> MNTINIAKNDFSDIELAAIPFNTLADHYGERLAREQLALEHESYEMGEARFRKMFERQLKAGEVADNAAAKPLITTLLPKMIARINDWFEEVKAKRGKRPTAFQFLQEIKPEAVAYITIKTTLACLTSADNTTVQAVASAIGRAIE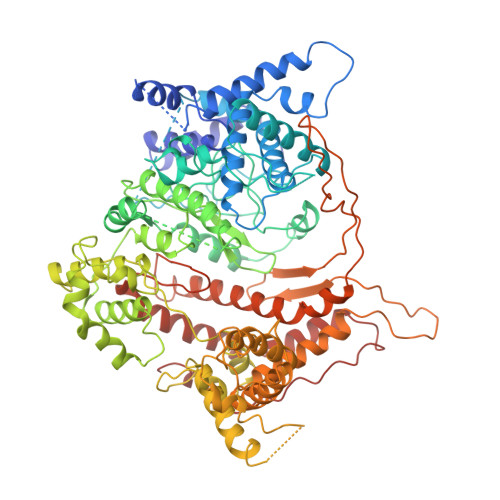DEARFGRIRDLEAKHFKKNVEEQLNKRVGHVYKKAFMQVVEADMLSKGLLGGEAWSSWHKEDSIHVGVRCIEMLIESTGMVSLHRQNAGVVGQDSETIELAPEYAEAIATRAGALAGISPMFQPCVVPPKPWTGITGGGYWANGRRPLALVRTHSKKALMRYEDVYMPEVYKAINIAQNTAWKINKKVLAVANVITKWKHSPVEDIPAIEREELPMKPEDIDMNPEALTAWKRAAAAVYRKDKARKSRRISLEFMLEQANKFANHKAIWFPYNMDWRGRVYAVSMFNPQGNDMTKGLLTLAKGKPIGKEGYYWLKIHGANCAGVDKVPFPERIKFIEENHENIMACAKSPLENTWWAEQDSPFCFLAFCFEYAGVQHHGLSYNCSLPLAFDGSCSGIQHFSAMLRDEVGGRAVNLLPSETVQDIYGIVAKKVNEILQADAINGTDNEVVTVTDENTGEISEKVKLGTKALAGQWLAYGVTRSVTKRSVMTLAYGSKEFGFRQQVLEDTIQPAIDSGKGLMFTQPNQAAGYMAKLIWESVSVTVVAAVEAMNWLKSAAKLLAAEVKDKKTGEILRKRSAVHWVTPDGFPVWQEYKKPIQTRLNLMFLGQFRLQPTINTNKDSEIDAHKQESGIAPNFVHSQDGSHLRKTVVWAHEKYGIESFALIHDSFGTIPADAANLFKAVRETMVDTYESSDVLADFYDQFADQLHESQLDKMPALPAKGNLNLRDILESDFAFA>[2x]HHHHHHSSGLVPRGSH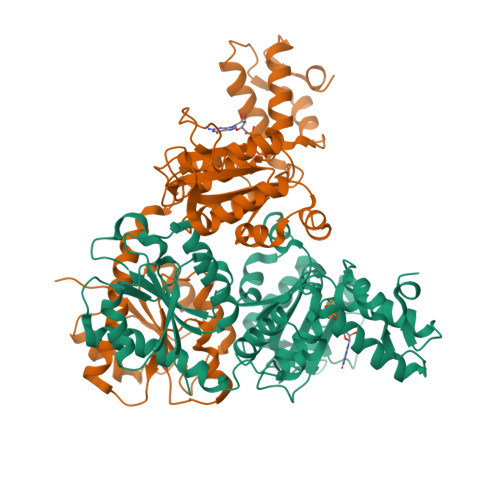MMSTQFRMDSVPGSLVVVGGTYEPWLPVLEKVGWRCTQVADLRKPDALFVETGPCIGIVDLSHDEFSLNGIANLVSSHKQVRWLAFIREAQLSSDTICQFIVNFCIDFFTAPIPDAQLLSTIGHQLGMLKLEKKVWPHFGSAGNMGLIGESMPMKRLRDQIKRIGPTDVSILIYGESGTGKETVAKAIHKTSSRAQKPFISVNCRAMSEKRLESELFGLGETEEGQQPFLLQADGGTLLLNDILTLPKSQQLNLLRFLQEGTVETRQGVRAVDVRILAANSSDIEKALIDGDFNEELYHYINVLRINVPSLKERASDIVLLAKHFLQEYSKEYNAQARSFSDDAVRGLTRYHWPGNVRELMNQIKRVVLMSDTVVLDESQLDL>GICGAGC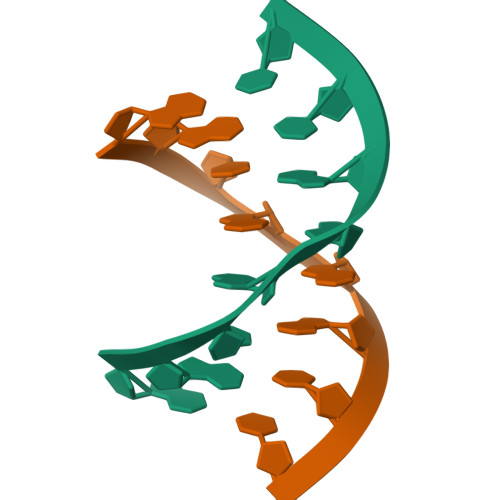C[5x]>SHEATVEYLA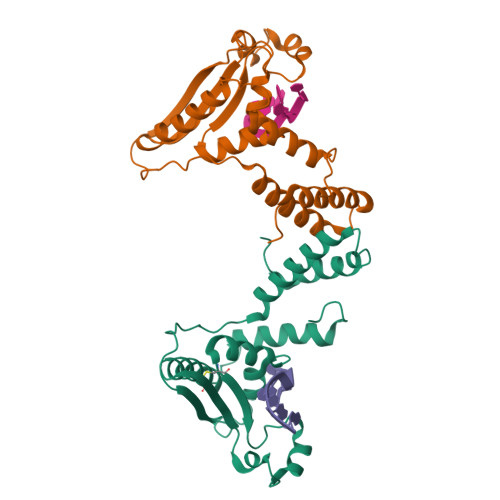DLVKEKKHLTLFPHMFSNVERLLDDEIGRVRVALFQTEFPRVELPEPAGDMISITEKIYVPKNEYPDYNFVGRILGPRGMTAKQLEQDTGCKIMVRGKGSMRDKSKESAHRGKANWEHLEDDLHVLVQCEDTENRVHIKLQAALEQVKKLLIPAPEGTDELKRKQLMELAIINGTYRPMKSPNPAR[2x]>MKKHHHHHHEQDTIPVSGSTGFDRGLEAEKILGASDNNGRLTFLIQFKGVDQAEMVPSSVANEKIPRMVIHFYEERLSWY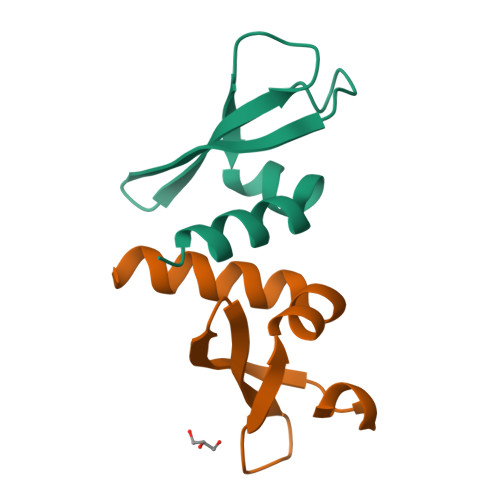SDNEDKK[2x]> GHGAPKAQKTGILLVAFGTSVEEARPALDKMGDRVRAAHPDIPVRWAYTAKMIRAKLRAEGIAAPSPAEALAGMAEEGFTHVAVQSLHTIPGEEFHGLLETAHAFQGLPKGLTRVSVGLPLIGTTADAEAVAEALVASLPADRKPGEPVVFMGHGTP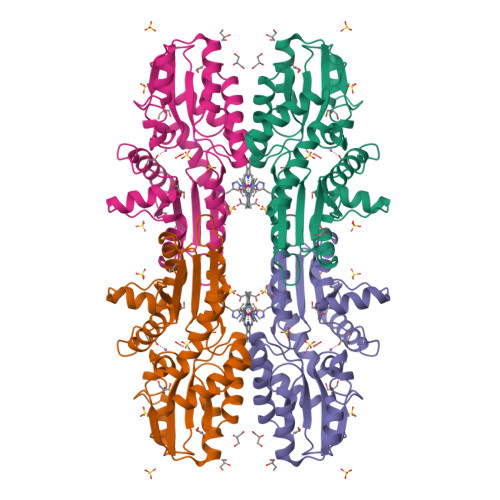HPADICYPGLQYYLWRLDPDLLVGTVEGSPSFDNVMAELDVRKAKRVWLMPLMAVAGDHARNDMAGDEDDSWTSQLARRGIEAKPVLHGTAESDAVAAIWLRHLDDALARLN> UGCUCCUAGUACGAGAGGACCGGAGUG

Atomic mutagenesis is the key to advance our understanding of RNA recognition and RNA catalysis. To this end, deazanucleosides are utilized to evaluate the participation of specific atoms in these processes. Here, we present the synthesis of this nucleoside and its phosphoramidite, allowing first time access to c1G-modified RNA. c1G is expected to impair Watson–Crick pairing because the central N1–H of G is replaced by C–H, thereby depriving the capability for the formation of strong hydrogen bonds.

To shed further light on the structural impact of c1G in RNA, we aimed at a high-resolution X-ray crystallographic analysis. We utilized the 27 nt fragment of the E. coli 23S rRNA sarcin/ricin loop (SRL), which is a frequently applied crystallization scaffold. For the replacement of G by c1G, we tested three different positions, including nucleotide G2669 which forms a Watson–Crick base pair with C2651 in the regular A-form double helical region, G2659 which forms a Hoogsteen pair with A2662 in the loop, and G2655 which interacts with the phosphate of G2664 in a bidentate fashion. From these three c1G-modified RNAs, only c1G2655-modified SRL RNA provided crystals that diffracted to atomic resolution (0.9 Å). X-ray structure determination demonstrated that the c1G nucleobase is well defined in the electron density maps for the c1G-modified RNA. The c1G-modified RNA structure superimposed with the unmodified RNA displayed a root-mean-square deviation (rmsd) of 0.09 Å (within the errors on coordinates of 0.09 Å). Direct comparison of the base triples U2656-A2665-G2655 and U2656-A2665-c1G2655 reveals that with the weakening (or loss) of the G2655 N1–H···O–P H-bond, c1G slightly opens up by retaining the H-bond between c1G2655 2-NH2 and O4 of U2656. A comparison of the melting profiles of wild-type and c1G modified SRL hairpins indicated a modest weakening of the fold. Taken together, our crystallization experiments imply that c1G does not significantly affect an RNA fold as long as it is not replacing G in a Watson–Crick base pair. The weakening (or loss) of an H-bond to the phosphate backbone seems better tolerated and allowed crystallization and structure solution.> AQPDIKFASKEYGVTIGESRIIYPLDAAGVMVSVKNTQDYPVLIQSRIYDENKEKESEDPFVVTPPLFRLDAKQQNSLRIAQAGGVFPRDKESLKWLCVKGIPPKDEDIWVDDATNKQKFNPDKDVGVFVQFAINNCIKLLVRPNELKGTPIQFAENLSWKVDGGKLIAENPSPFYMNIGELTFGGKSIPSHYIPPKSTWAFDLPKGLAGARNVSWRIINDQGGLDRLYSKNVTL;>ADLTASTTVTVTVVEPARITLTYKEGAPITIMDNGNIDTELLVGTLTLGGYKTGTTSTSVNFTDAAGDPMYLTFTSQDGNNHQFTTKVIGKDSRDFDISPKVNGENLVGDDVVLATGSQDFFVRSIGSKGGKLAAGKYT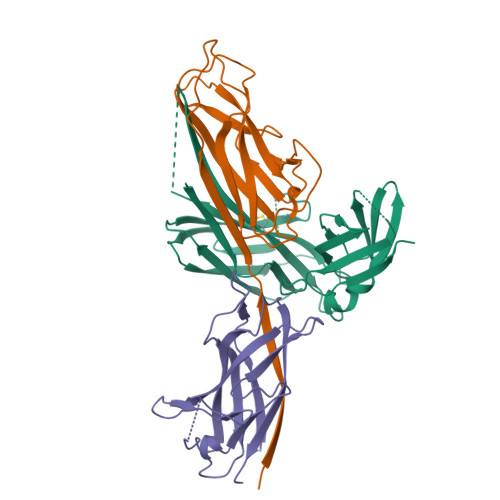DAVTVTVSNQ[2x]> MGVIKKKRSHHGKASRQQYYSGVQVGGVGSMGAINNNIPSLTSFAEENNYQYGYSGSSAGMNGRSLTYAQQQLNKQRQDFERVRLRPEQLSNIIHDESDTISFRSNLLKNFISSNDAFNMLSLTTVPCDRIEKSRLFSEKTIRYLMQKQHEMKTQAAELQEKPLTPLKYTKLIAAAEDGSRSTKDMIDAVFEQDSHLRYQPDG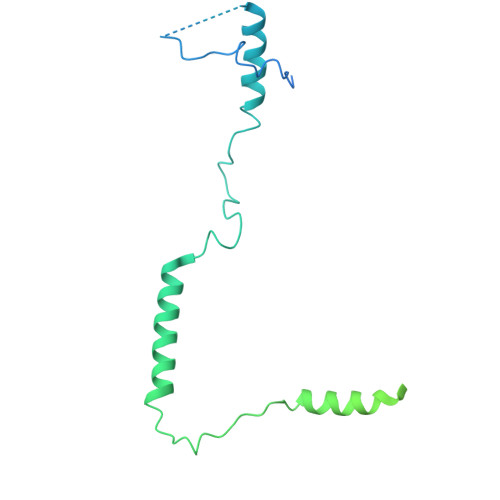VVVHRDDPALVGKLRGDLREAPADYWTHAYRDVLAQYHEAKERIRQKEVTAGEAQDEASLQQQQQQDLQQQQQVVTTVASQSPHATATEKEPVPAVVDDPLENMFGDYSNEPFNTNFDDEFGDLDAVFF>MPIATPEVYAEMLGQAKQNSYAFPAINCTSSETVNAAIKGFADAGSDGIIQFSTGGAEFGSGLGVKDMVTGAVALAEFTHVIAAKYPVNVALHTDHCPKDKLDSYVRPLLAISAQRVSKGGNPLFQSHMWDGSAVPIDENLAIAQELLKAAAAAKIILEIEIGVVGGEEDGVANEINEKLYTSPEDFEKTIEALGAGEHGKYLLAATFGNVHGVYKPGNVKLRPDILAQGQQVAAAKLGLPADAKPFDFVFHGGSGSLKSEIEEALRYGVV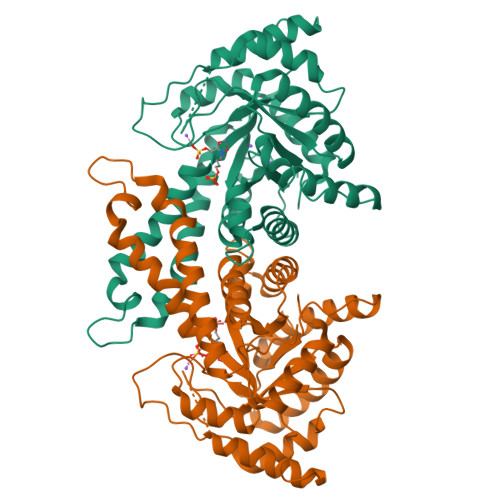KMNVDTDTQYAFTRPIAGHMFTNYDGVLKVDGEVGVKKVYDPRSYLKKAEASMSQRVVQACNDLHCAGKSLTH[4x]> EIPV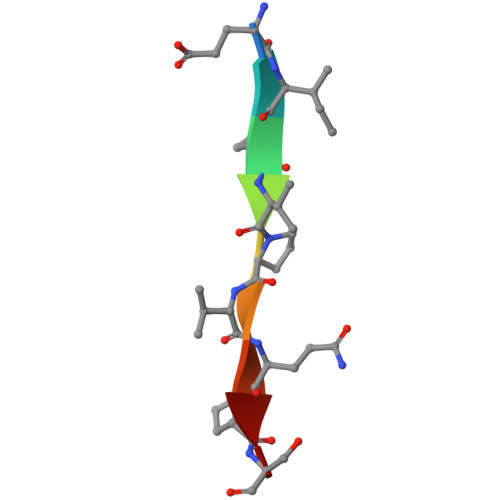PVQPS>AMATAPRPLREQYLHFQPISTRWHDNDIYGHVNNVTYYAFFDTAVNTYLIERGGLDIQGGEVIGLVVSSSCDYFAPVAFPQRIEMGLRVARL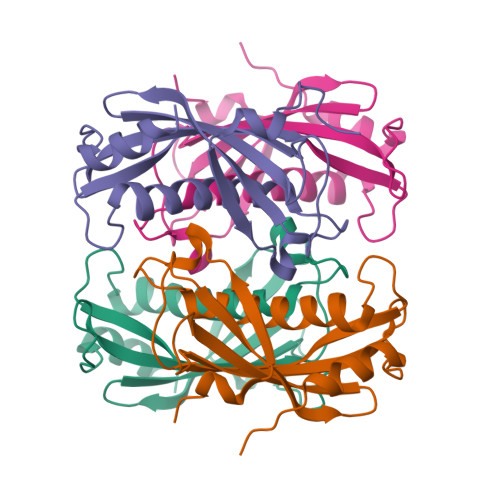GNSSVQYELALFLEGQREACAAGRFVHVFVERRSSRPVAIPQELRDALAALQSSAQ[3x]>[2x]GGHHHHHHGSENLYFQGACPSQCSCSGTTVDCSGKSLASVPGGIPTTTQVLYLYDNQITKLEPGVFDRLVNLQQLWLEINQLTSLPAGVFDNLTQLSILNMHTNQLKSIPRGAFD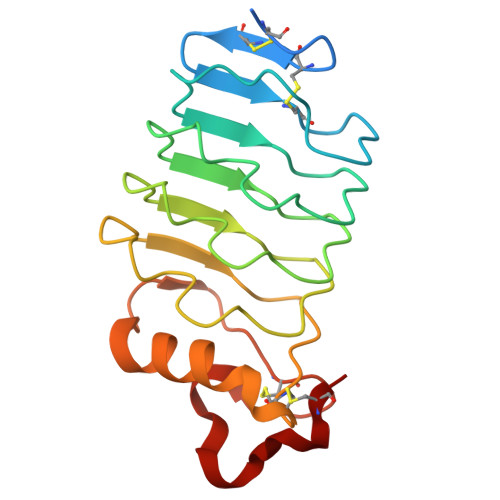NLKSLTHIWLLNNPWDCACSDILYLSGWLGQHAGKEQGQAVCSGTNTPVRAVTEASTSPSKCP> MGHMNITDIREQFPILHQQVNGHDLVYLDSAATSQKPRAVIETLDKYYNQYNSNVHRGVHTLGTRATDGYEGAREKVRKFINAKSMAEIIFTKGTTTSLNMVALSYARANLKPGDEVVITYMEHHANIIPWQQAVKATGATLKYIPLQEDGTISLEDVRETVTSNTKIVAVSHVSNVLGTVNPIKEMAKIAHDNGAVIVVDGAQSTPHMKIDVQDLDCDFFALSSHKMCGPTGVGVLYGKKALLENMEPAEFGGEMIDFVGLYESTWKELPWKFEAGTPIIAGAIGLGAAIDFLEEIGLDEISRHEHKLAAYALERFRQLDGVTVYGPEERAGLVTFNLDDVHPHDVATVLDAEGIAVRAGHHCAQP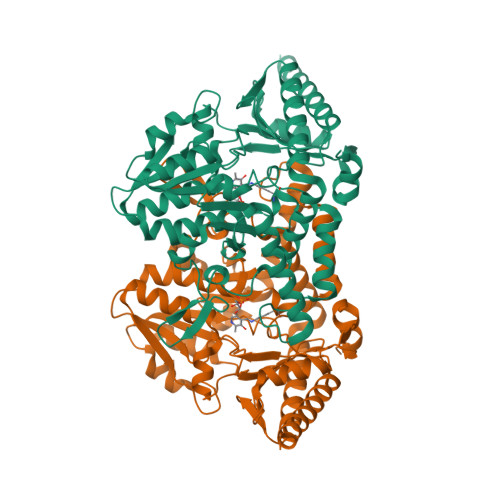LMKWLDVTATAAASFYLYNTEEEIDKLVEALQKTKEYFTNVFVDLEHHHHHH> EPSERCDDWGLDTMRQIQVFEDEPARIKCPLFEHFLKFNYSTAH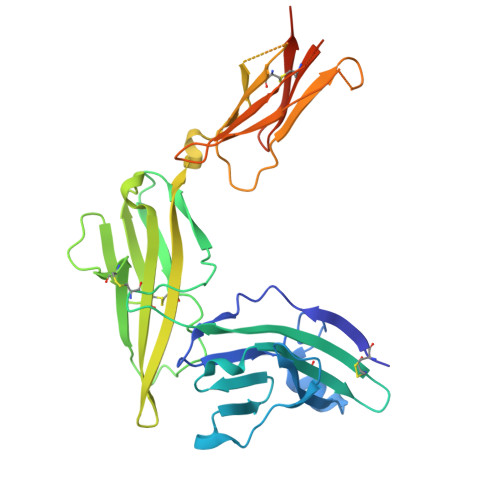SAGLTLIWYWTRQDRDLEEPINFRLPENRISKEKDVLWFRPTLLNDTGNYTCMLRNTTYCSKVAFPLEVVQKDSCFNSPMKLPVHKLYIEYGIQRITCPNVDGYFPSSVKPTITWYMGCYKIQNFNNVIPEGMNLSFLIALISNNGNYTCVVTYPENGRTFHLTRTLTVKVVGSPKNAVPPVIHSPNDHVVYEKEPGEELLIPCTVYFSFLMDSRNEVWWTIDGKKPDDITIDVTINESISHSRTEDETRTQILSIKKVTSEDLKRSYVCHARSAKGEVAKAAKVKQKVPAPRYTVELACGFGAT>[2x]GSHMASMLLDTFQGYNCYSSALGEYAKQKNIDQVENIILSQWSFFFDEEQFYKNQWYTGAADGPVDVVLNEDLRNFANIEVLEHISSESQAIDEGRKVLEKHGLQIVLMDFYYMNSFNWKSLSRFNVTREHDPAFAVLTQINENSVHIIDPYYHHEENMSMEDFIKSRNSMTKQGKISFNSYEIFSNGTKKSNI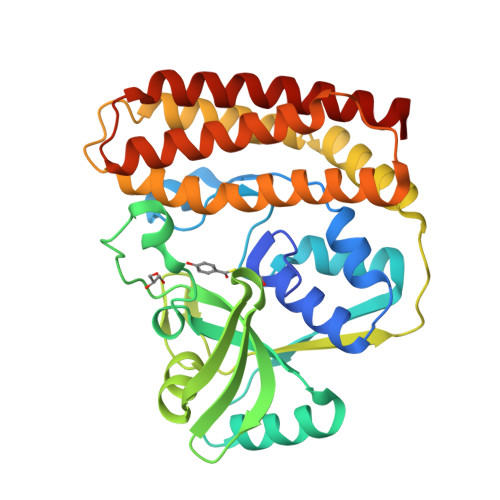KELLYYRFNRYLQEKMFGKITQFGQVVKKQLDNKDRKWAFTGYNCLNSVVYQHQNLINLQKKFSLEMPPNLQELLDNWALIRKKLFEYYSRGSYNTEEISNLICKVASSEEQFAQEVLKVL4-bromo-6-[(3,4-dichlorophenyl)sulfanyl]-1-{[4-(dimethylcarbamoyl)phenyl]methyl}-1H-indole-2-carboxylic acid | C25 H19 Br Cl2 N2 O3 S | 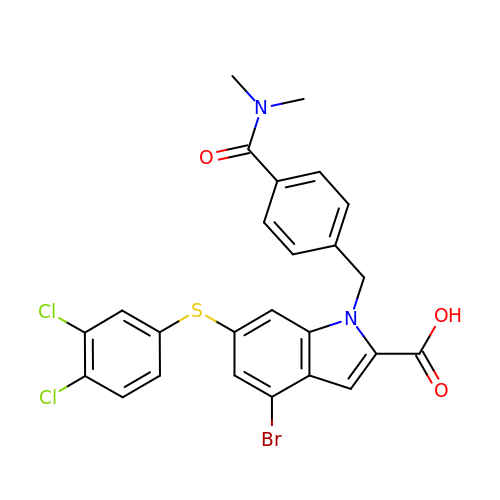MJYFVDNMTKLGTH-UHFFFAOYSA-N> MNLFQTVFTGSKQALAAAEGIVKQAVDEKGRDYKVAFPDTAYSLPVIFAATGKKITNVGELEGALDIVRSLIVEEEMLDKLLNSGLATAVAAEIIEAAKYVLSDAPYAEPCVGFISDPIIRSLGVPLVTGDIPGVAVILGECPDSETAAKIIKDYQSKGLLTCLVGKVIDQAIEGKVKMGLDLRVIPLGYDVTSVIHVVTIAIRAALIFGGIKGGQLNDILKYTAERVPAFVNAFGPLSELVVSAGAGAIALGFPVLTDQVVPEVPTLLLTQKDYDKMVKTSLEARNIKIKITEIPIPVSFAAAFEGERIRKNDMLAEFGGNKTKAWELVMCADQGEVEDHKIEVIGPDIDTIDKAPGRMPLGMLIKVSGTNMQKDFEPVLERRLHYFLNYIEGVMHVGQRNLTWVRIGKEAFEKGFRLKHFGEVIYAKMLDEFGSVVDKCEV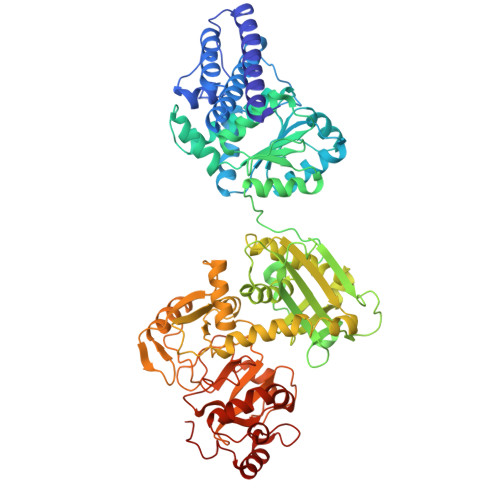TIITDPGKAEELEGKYAVPRYKERDARLESLVDEKVDTFYSCNLCQSFAPAHVCIVTPERLGLCGAVSWLDAKATLELNPTGPCQAVPKEGVVDENLGIWEKVNETVSKISQGAVTSVTLYSILQDPMTSCGCFECITGIMPEANGVVMVNREFGATTPLGMTFGELASMTGGGVQTPGFMGHGRQFIASKKFMKGEGGLGRIVWMPKELKDFVAEKLNKTAKELYNIDNFADMICDETIATESEEVVKFLEEKGHPALKMDPIM>[2x]DENSKKTQELVEKLPHEVLELYKNVGGEIYITDKRLTQHEELSDSSHKDMFIVSSEGKSFPLREHFVFAKGGKEPSLIIHAEDYASHLSSVEVYYELGKAIIRDTFPLNQKELGNPKFINAINEVNQQKEGKGVNAKADEDGRDLLFGKELKKNLEHGQLVDLDLISGNLSEFQHVFAKSFALYYEPHYKEALKSYAPALFNYMLE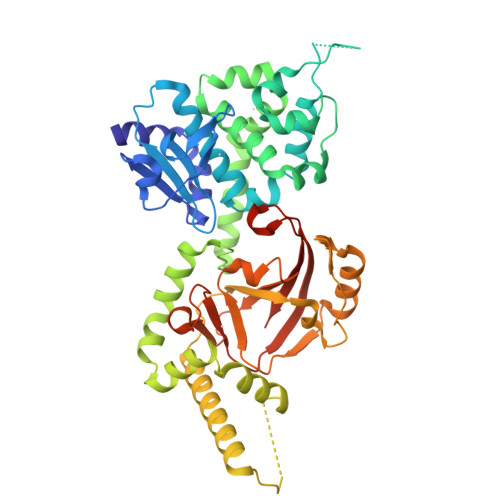LDQMRFKEISDDVKEKNKNVLDFKWYTRKAESWGVQTFKNWKENLTISEKDIITGYTGSKYDPINEYLRKYDGEIIPNIGGDLDKKSKKALEKIENQIKNLDAALQKSKITENLIVYRRVSELQFGKKYEDYNLRQNGIINEEKVMELESNFKGQTFIQHNYMSTSLVQDPHQSYSNDRYPILLEITIPEGVHGAYIADMSEYPGQYEMLINRGYTFKYDKFSIVKPTREEDKGKEYLKVNLSIYLGNHHHHHH>[12x]MTTVLPPLEDTDGLWAALTEAAASVEKLLA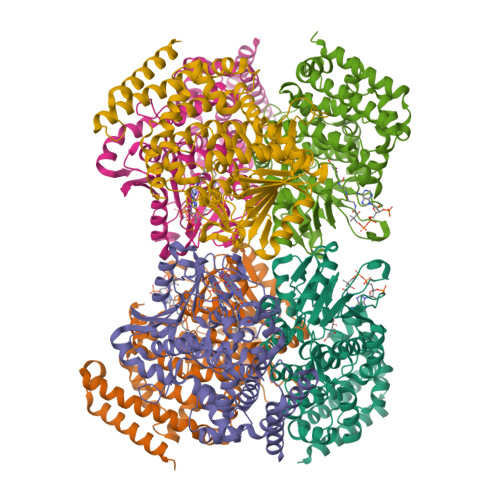TLPEHGARSSAERAEIAAAHDAARALRVRFLDTHADAVYDRLTDHRRVHLRLAELVEAAATAFPGLVPTQQQLAVERSLPQAAKEGHEIDQGIFLRAVLRSPLAGPHLLDAMLRPTPRALELLPEFVRTGEVEMEAVHLERRDGVARLTMCRDDRLNAEDGQQVDDMETAVDLALLDPGVRVGLLRGGVMSHPRYRGKRVFSAGINLKYLSQGGISLVDFLMRRELGYIHKLVRGVLTNDDRPGWWHSPRIEKPWVAAVDGFAIGGGAQLLLVFDRVLASSDAYFSLPAAKEGIIPGAANLRLGRFAGPRVSRQVILEGRRIWAKEPEARLLVDEVVEPDELDAAIERSLTRLDGDAVLANRRMLNLADESPDGFRAYMAEFALMQALRLYGHDVIDKVGRFGGRPPA>MQTAEQNPLRLGVQLYALGRYDAALTLFERALKENPQDPEALYWLARTQLKLGLVNPALENGKTLVARTPRYLGGYMVLSEAYVALYRQAEDRERGKGYLEQALSVLKDAERVNPRYAPLHLQRGLVYALLGERDKAEASLKQALALEDTPEIRSALAELYLSMGRLDEALAQYAKALEQAPKDLDLRVRYASALLLKGKAEEAARAAALEHH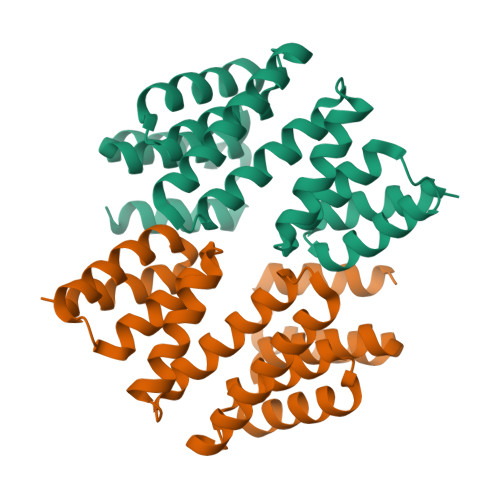HHHH[2x]>RDMPLDSDVFRVPPGYNAPQQVHITQGDLVGRAMIISWVTMDEPGSSAVRYWSEKNGRKRIAKGKMSTYRFFNYSSGFIHHTTIRKLKYNTKYYYEVGLRNTTRRFSFITPPQTGLDVPYTFGLIGDLGQSFDSNTTLSHYELSPKKGQTVLFVGDLSYADRYPNHDNVRWDTWGRFTERSVAYQPWIWTAGNHEIEFAPEINETEPFKPFSYRYHVPYEASQSTSPFWYSIKRASAHIIVLSSYSAYGRGTPQYTWLKKELRKVKRSETPWLIVLMHSPLYNSYNHHFMEGEAMRTKFEAWFVKYKVDVVFAGHVHAYERSERVSNIAYKITNGLCTPVKDQSAPVYITIGDAGNYGVIDSNMIQPQPEYSAFREASFGHGMFDIKNRTHAHFSWNRNQDG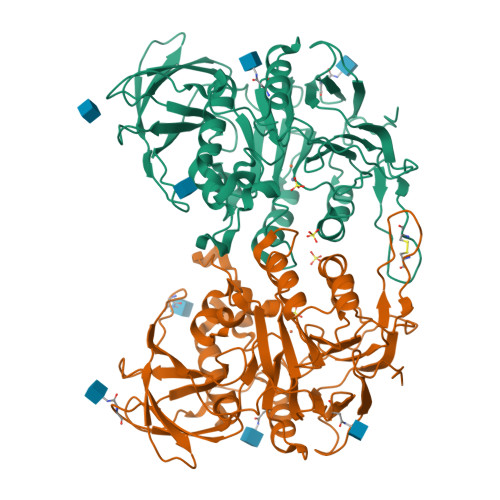VAVEADSVWFFNRHWYPVDDST[2x]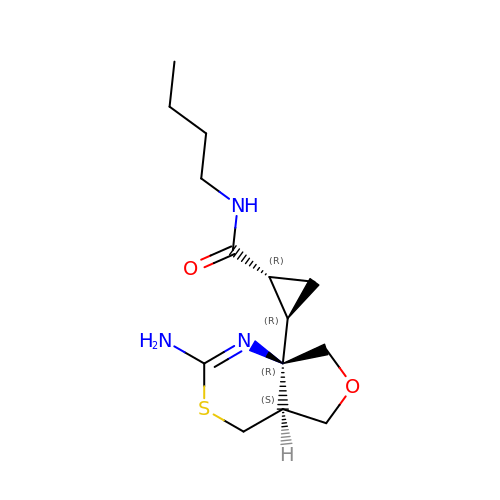(1R,2R)-2-[(4aS,7aR)-2-amino-4a,5-dihydro-4H-furo[3,4-d][1,3]thiazin-7a(7H)-yl]-N-butylcyclopropane-1-carboxamide | C14 H23 N3 O2 S | WVAFMFLAAGBATC-OXIWPEFWSA-N Here, we investigate the capability of a deep neural network model to automate design of sequences onto protein backbones, having learned directly from crystal structure data and without any human-specified priors. To assess whether the model could perform sequence design for de novo structures, we tested our method on a Rosetta-generated four-fold symmetric de novo TIM-barrel backbone, a (βαβα)4 topology consisting of an eight-stranded barrel surrounded by eight alpha helices. We had the model fully redesign 50 four-fold symmetric sequences for the backbone and selected 8 designs for further characterization based on ranking by the model PLL and other metrics (see “Methods” section), using no information about previously confirmed sequences. Of these 8 designs, 4 are cooperatively folded proteins, as indicated by circular dichroism (CD) wavelength scans and by the presence of clear two-state transitions in thermal melt curves.

We successfully crystallized 2 model designs, F2C (1.46 Å resolution) and F15C (1.9 Å resolution), and the crystal structures validate that the sequences indeed fold into the TIM-barrel structure in agreement with the designed backbone. F15C adopts the full TIM-barrel fold, but for two of four monomers in the asymmetric unit of F15C, one of the β-α loops shifts to interact with an adjacent monomer in the crystal. However, we note that F15C primarily elutes as a monomer in size exclusion chromatography, and the interactions observed in the crystal structure resemble crystal packing, rather than a stable dimer interface. For F2C, the model uses an isoleucine to wedge between the long and short helices and forming a Tyr-Glu-Ser polar network that extends to coordinate the loop from the beta-sheet to the short helix; for F15C, the model has a different solution, designing phenylalanine and valine residues (F10, V14) to pack the long helix against the shorter one near the top of the barrel. Particularly interesting are the Tyr-backbone contact and the His-Glu-backbone polar network for F2C and F15C, respectively, that help coordinate the helices across symmetric subunits at the base of the structure; these are the only hydrogen bonding solutions designed at this position among all previous structure-confirmed sequences for this scaffold. All of the folded proteins designed by our model have higher thermal stability than the initial designs reported in the original study, with melting temperatures for 3 of the 4 ranging between 84 and 87 °C while the fourth protein (F5C) remains folded at 95 °C.

>MDILIVNPDDFEKGVEEVKELKRHGAKIIAYISKSAEELKKAEKAGADILIVNPDDFEKGVEEVKELKRHGAKIIAYISKSAEELKKAEKAGADILIVNPDDFEKGVEEVKELKRHGAKIIAYISKSAEELKKAEKAGADILIVNPDDFEKGVEEVKELKRHGAKIIAYISKSAEELKKAEKAG[4x]2-fluoro-N-[(1H-pyrazol-3-yl)methyl]aniline | C10 H10 F N3 | 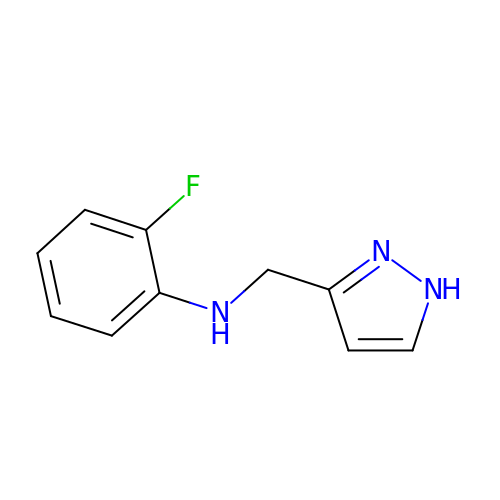IREDHAFKGFKXRR-UHFFFAOYSA-N6-[5-({(3R,4R)-4-[(6-amino-4-methylpyridin-2-yl)methyl]pyrrolidin-3-yl}oxy)pentyl]-4-methylpyridin-2-amine 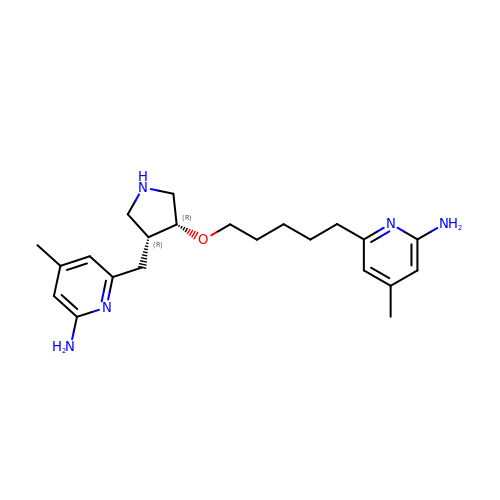| C22 H33 N5 O | WKAYHKZPKWNKSL-XLIONFOSSA-N> GAMEDEMPKT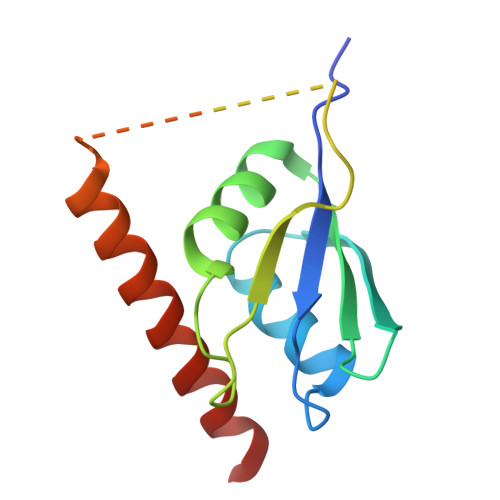LYVGNLSRDVTEALILQLFSQIGPCKNCKMIMDTAGNDPYCFVEFHEHRHAAAALAAMNGRKIMGKEVKVNWATTPSSQKKDTSGSGGSGGSGGSGGSGHKENVKDYYQKWMEEQAQSLIDKTTAAFQQGK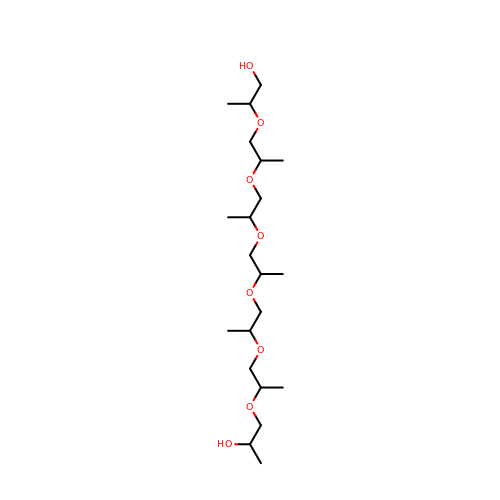(20S)-2,5,8,11,14,17-HEXAMETHYL-3,6,9,12,15,18-HEXAOXAHENICOSANE-1,20-DIOL | C21 H44 O8 | OWRNLGZKEZSHGO-QAWAPDBNSA-N[(6-oxo-4-phenyl-1,6-dihydropyrimidin-2-yl)sulfanyl]acetic acid | C12 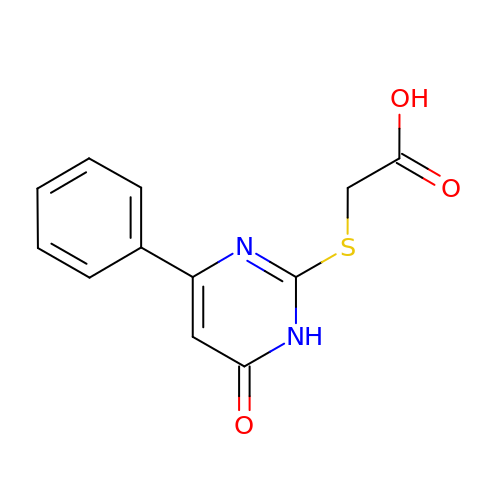H10 N2 O3 S | NVFIGQYDZXKAEK-UHFFFAOYSA-N> MI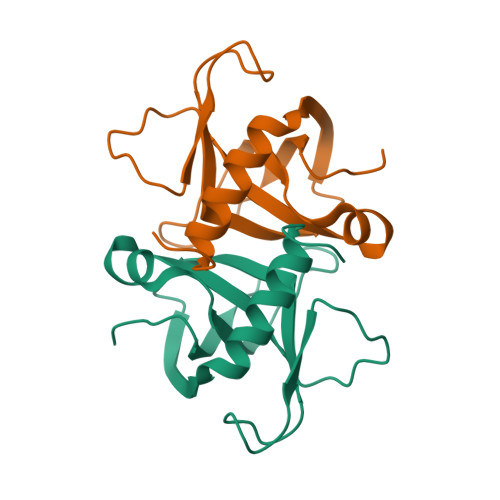VKRGDVYFADLSPVVGSEQGGVRPVLVIQNDIGNRFSPTVIVAAITAQIQKAKLPTHVEIDAKKYGFERDSVILLEQIRTIDKQRLTDKITHLDEVMMIRVDEALQISLGLIDF> PISPIETVPVKLKPGMDGPKVKQWPLTEEKIKALVEICTEMEKEGKISKIGPENPYNTPVFAIKKKDSTKWRKLVDFRELNKRTQDFWEVQLGIPHPAGLKKKKSVTVLDVGDAYFSVPLDEDFRKYTAFTIPSINNETPGIRYQYNVLPQGWKGSPAIFQSSMTKILEPFKKQNPDIVIYQYMDDLYVGSDLEIGQHRTKIEELRQHLLRWGLTTPDKKHQKEPPFLWMGYELHPDKWTVQPIVLPEKDSWTVNDIQKLVGKLNWASQIYPGIKVRQLCKLLRGTKALTEVIPLTEEAELELAENREILKEPVHGVYYDPSKDLIAEIQKQGQGQWTYQIYQEPFKNLKTGKYARMRGAHTNDVKQLTEAVQKITTESIVIWGKTPKFKLPIQKETWETWWTEYWQATWIPEWEFVNTPPLVKLWYQLEKEPIVGAETFYVDGAANRETKLGKAGYVTNKGRQKVVPLTNTTNQKTELQAIYLALQDSGLEVNIVTDSQYALGIIQAQPDKSESELVNQIIEQLIKKEKVYLAWVPAHKGIGGNEQVDKLVSAGIR;> PISPIETVPVKLKPGMDGPKVKQWPLTEEKIKALVEICTEMEKEGKISKIGPENPYNTPVFAIKKKDS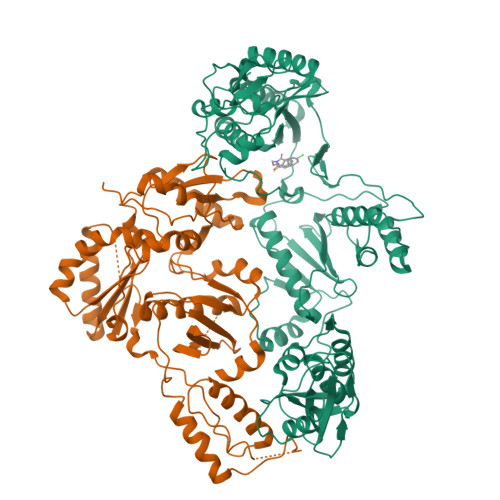TKWRKLVDFRELNKRTQDFWEVQLGIPHPAGLKKKKSVTVLDVGDAYFSVPLDEDFRKYTAFTIPSINNETPGIRYQYNVLPQGWKGSPAIFQSSMTKILEPFKKQNPDIVIYQYMDDLYVGSDLEIGQHRTKIEELRQHLLRWGLTTPDKKHQKEPPFLWMGYELHPDKWTVQPIVLPEKDSWTVNDIQKLVGKLNWASQIYPGIKVRQLCKLLRGTKALTEVIPLTEEAELELAENREILKEPVHGVYYDPSKDLIAEIQKQGQGQWTYQIYQEPFKNLKTGKYARMRGAHTNDVKQLTEAVQKITTESIVIWGKTPKFKLPIQKETWETWWTEYWQATWIPEWEFVNTPPLVKLWYQ>[12x]MAINFKGSPYLDRFDPSKDRTKVLFNPDRPLQQAELNEMQSIDQYYLKNLGDAIFKDGDKQSGLGFTLSEDNVLTVNPGYVYINGKIRYYDNDDSVKITGVGKETIGIKLTERIVTPDEDASLLDQTSGVPSYFSKGADRLEEKMSLTVNDPTSATIYTFMDGDLYIQSTNAEMDKINKVLAERTYDESGSYKVNGFELFSEGNAEDDDHVSVVVDAGKAYVKGFKVDKPVSTRISVPKSYDLGTAENESTIFNKSNNSISLANSPVKEIRRVTGQVLIEKERVTRGAQGDGQDFLSNNTAFEIVKVWTETSPGVTTKEYKQGEDFRLTDGQTIDWSPQGQEPSGGTSYYVSYKYNKRMEAGKDYEVTTQGEGLSKKWYINFTPSNGAKPIDQTVVLVDYTYYLARKDSVFINKYGDIAILPGEPNIMRLVTPPLNTDPENLQLGTVTVLPDSDEAVCISFAITRLSMEDLQKVKTRVDNLEYNQAVNALDDGAMEGQNPLTLRSVFSEGFISLDKADITHPDFGIVFSFEDAEATLAYTEAVNQPKIIPGDTTAHIWGRLISAPFTEERTIYQGQASETLNVNPYNIPNKQGVLKLTPSEDNWIDTENVTITEQKTKKVTMKRFWRHNESYYGETEHYLYSNLQLDAGQKWKGETYAYDREHGRTGTLLESGGQRTLEEMIEFIRIRDVSFEVKGLNPNDNNLYLLFDGVRCAITPATGYRKGSEDGTIMTDAKGTAKGKFTIPAGIRCGNREVTLKNANSTSATTYTAQGRKKTAQDIIIRTRVTVNLVDPLAQSFQYDENRTISSLGLYFASKGDKQSNVVIQIRGMGDQGYPNKTIYAETVMNADDIKVSNNASAETRVYFDDPMMAEGGKEYAIVIITENSDYTMWVGTRTKPKIDKPNEVISGNPYLQGVLFSSSNASTWTPHQNSDLKFGIYTSKFNETATIEFEPIKDVSADRIVLMSTYLTPERTGCTWEMKLILDDMASSTTFDQLKWEPIGNYQDLDVLGLARQVKLRATFESNRYISPLMSSSDLTFTTFLTELTGSYVGRAIDMTEAPYNTVRFSYEAFLPKGTKVVPKYSADDGKTWKTFTKSPTTTRANNEFTRYVIDEKVKSSGTNTKLQVRLDLSTENSFLRPRVRRLMVTTRDE;>[6x]MALNFTTITENNVIRDLTTQVNNIGEELTKERNIFDITDDLVYNFNKSQKIKLTDDKGLTKSYGNITALRDIKEPGYYYIGARTLATLLDRPDMESLDVVLHVVPLDTSSKVVQHLYTLSTNNNQIKMLYRFVSGNSSSEWQFIQGLPSNKNAVISGTNILDIASPGVYFVMGMTGGMPSGVSSGFLDLSVDANDNRLARLTDAETGKEYTSIKKPTGTYTAWKKEFEPKDMEKYLLSSIRDDGSASFPLLVYTSDSKTFQQAIIDHIDRTGQTTFTFYVQGGVSGSPMSNSCRGLFMSDTPNTSSLHGVYNAIGTDGRNVTGSVVGSNWTSPKTSPSHKELWTGAQSFLSTGTTKNLSDDISNYSYVEVYTTHKTTEKTKGNDNTGTICHKFYLDGSGTYVCSGTFVSGDRTDTKPPITEFYRVGVSFKGSTWTLVDSAVQNSKTQYVTRIIGINMP;>MAFNYTPLTETQKLKDMYPKVNDIGNFLKTEVNLSDVKQISQPDFNNILASIPDSGNYYVTNSKGAPSGEATAGFVRLDKRNVNYYKIYYSPYSSNKMYIKTYANGTVYDWISFKLDEGSLYNEGNTLNVKELTESTTQYATLVNPPKENLNTGWVNYKESKNGVSSLVEFNPVNSTSTFKMIRKLPVQEQKPNLLKDSLFVYPETSYSNIKTDNWDTPPFWGYSSNSGRSGVRFRGENTVQIDDGSDTYPSVVSNRFKMGKELSVGDTVTVSVYAKINDPALLKDNLVYFELAGYDTVDDTSKNPYTGGRREITASEITTEWKKYSFTFTIPENTIGASGVKVNYVSLLLRMNCSSSKGNGAVVYYALPKLEKSSKVTPFITHENDVRKYDEIWSNWQEVISKDELKGHSPVDIEYNDYFKYQWWKSEVNEKSLKDLAMTVPQGYHTFYCQGSIAGTPKGRSIRGTIQVDYDKCDPYRANKFVKLLFTDTEGIPYTLYYGGYNQGWKPLKQSETSTLLWKGTLDFGSTEAVNLNDSLDNYDLIEVTYWTRSAGHFSTKRLDIKNTSNLLYIRDFNISNDSTGSSVDFFEGYCTFPTRTSVQPGMVKSITLDGSTNTTKVASWNEKERIKVYNIMGINRG[6x];> MATDKEAKDVIDKFIDNVFNFDVLTKERIKEKDEEIKKITTDDMYEKVVYIRPYVGVIQSLNPQHVQYESFSNNGYDIEAELSFRKVSYLVDKGSIPTDSLSTLTVHLVERNQELLIDYFDEIQDVLYGEYMEEEYVFDEDVPLSTILALDLNDNLKSLSNIKYMFKGAPKENPFGTDKDVYIDTYNLLYWLYLGEDEELAYPMNINYFFTEGRFFTIFGKGHKYKVDVSKFIVGDILFFGRSDTNIGIYVGDGEFISMMGKFPKDETPIGKYKLDDYWNEFNGRVMRFDEEVYI;> MVVRFQSSMGRSLKRVDSD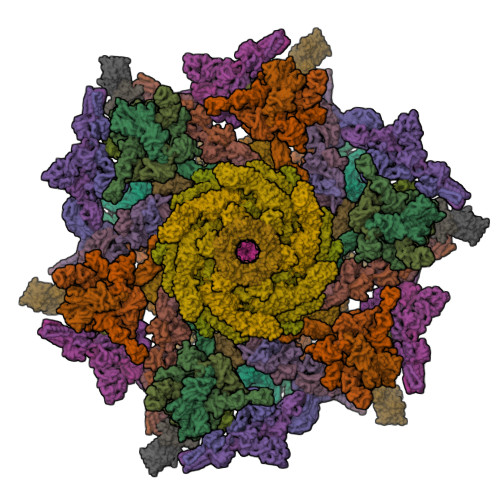DLNVKGLVLATVSKINYKYQSVEVKVNNLTLGSRIGDDGSLAVPYPKSFIGRTPEGSVFGTKPLITEGSVVLIGFLNDDINSPIILSVYGDNEQNKMINTNPLDGGKFDTESVYKYSSSLYEILPSLNYKYDDGEGTSIRTYNGKSFFSMTSGEEEKPQATDFYTGTEYQDLFTSYYGNKTLIEPRIQKAPNMLFKHQGVFYDDGTPDNHITTLFISERGDIRASVLNTETQKRTTQEMSSDGSYRVIKQDDDLMLDEAQVWIEYGISEDNKFYIKNDKHKFEFTDEGIYIDDKPMLENLDESIAEAMKNLNEIQKELDDINYLLKGVGKDNLEELIESTKESIEASKKATSDVNRLTTQIAEVSGRTEGIITQFQKFRDETFKDFYEDASTVINEVNQNFPTMKTDVKTLKTKVDNLEKTEIPNIKTRLTELENNNNNADKIISDRGEHIGAMIQLEENVTVPMRKYMPIPWSKVTYNNAEFWDSNNPTRLVVPKGITKVRVAGNVLWDSNATGQRMLRILKNGTYSIGLPYTRDVAISTAPQNGTSGVIPVKEGDYFEFEAFQDSEGDRQFRADPYTWFSIEAIELETETMEKDFMLIGHRGATGYTDEHTIKGYQMALDKGADYIELDLQLTKDNKLLCMHDSTIDRTTTGTGKVGDMTLSYIQTNFTSLNGEPIPSLDDVLNHFGTKVKYYIETKRPFDANMDRELLTQLKAKGLIGIGSERFQVIIQSFARESLINIHNQFSNIPLAYLTSTFSESEMDDCLSYGFYAIAPKYTTITKELVDLAHSKGLKVHAWTVNTKEEMQSLIQMGVDGFFTNYLDEYKKI;>MKTRKLTNILSKLIDKTMAGTSKITDFTPGSASRSLLEAVSLEIEQFYILTKENIDWGIQEGIIEAFDFQKRQSKRAYGDVTIQFYQPLDMRMYIPAGTTFTSTRQEYPQQFETLVDYYAEPDSTEIVVEVYCKETGVAGNVPEGTINTIASGSSLIRSVNNEYSFNTGTKEESQEDFKRRFHSFVESRGRATNKSVRYGALQIPDVEGVYVYEETGHITVFAHDRNGNLSDTLKEDIIDALQDYRPSGIMLDVTGVEKEEVNVSATVTISNKSRIGDTLQKHIESVIRSYLNNLKTSDDLIITDLIQAIMNIDDVLIYDVSFDNLDENIIVPPQGIIRAGEIKVELK[4x];> MRRIRRPKVRIEIVTDDNTFTLRFEDTRDYNGDEFGAKLLGFQTKNSMEDDSSVFQINMAGDTYWDKLVMANDIIRIFITPNDDPNDKEGKQERLIQVGMVSQVSKVGSYGNDQTQFRITGQSFVKPFMKFGLGVIQEVQAVLPEVGWLIDGDGDNEVKFTGSSAHEVMTGIIRRFIPYMKYNYTEKTYNTIDNYLDYDDLSSWDEFEKLTEVSAFTNFDGSLKQLMDMVTARPFNELFFKNSEKTPGKAQLVLRKTPFNPTEWRALDMIKVPTEDFIEEDVGKSDVETYSIFTATPAGMLKELNGDVFSKPQFHPELTDRYGYTKFEVENIYLSTKSGSATEDSDSSGDDNGTERGTYSKIMKDLSNYGRDNISKGIDKYTSKLSSKYKNLKKAQAKKIIEKFVKEGKVTEKEYEKITGNKVDDELTSDNRPKLTKDKLKSILKEKFKTQDDFNNSKKKKKAKTDALKELTTKYRFGNKTHATTLLDEYIKYKGEPPNDEAFDKYLKAIEGVSNVATDTGSDASDSPLVMFSRMLFNWYHGNPNFYAGDIIVLGDPKYDLGKRLFIEDKQRGDTWEFYIESVEHKFDYKQGYYTTVGVTRGLKDAILEDGKGSPHRFAGLWNQSSDFMGGLMGEDTSKELKEKGVAEKQSSGDKDGGSDSGGAQDGGSLDSLKKYNGKLPKHDPSFVQPGNRHYKYQCTWYAYNRRGQLGIPVPLWGDAADWIGGAKGAGYGVGRTPKQGACVIWQRGVQGGSPQYGHVAFVEKVLDGGKKIFISEHNYATPNGYGTRTIDMSSAIGKNAQFIYDKK;>MNNFIPQPQGLLRFLNTLDTDLTSSHMNLLDEEVSFVSKFYTPQLQLSELAKKVLTNIKTDDIPVLEREFNDNTIIHKANDTLLKVQAPRMYMILQSIVLEAYAIVNCFVENPSSLKYLTEEDVSITRENLNYVADYLGNYDDYNSVVLDLRDLDLCFSAIELQLPLIKKEANV[2x];>[2x]MANFLKNLHPLLRRDRNKKDNQDPNFALIDALNEEMNQVEKDAIESKLQSSLKTSTSEYLDKFGDWFGVYRKTDEKDDVYRARIIKYLLLKRGTNNAIIDAIKDYLGRDDIDVSVYEPFTNIFYTNKSHLNGEDHLMGYYYRFAVINVSIGDYFPVEIIDVINEFKPAGVTLYVTYDGASTIRGGAIIKWLDGLPKIETYQEFDRFTGYDDTFYGHINMNQSKDTDNSSSDIFKTNHSLINSLDVLTGSSSVGRQYINYGYVTSYVYNPGMTSSVNQISASTEGRGQEVPTDYYMYTSTKNNNTVELSMQTTSGVSYLYNNFNFRDYMSKYRPQVDLQSDEARRIVSDYIKELSIDYYLSAVIPPDESIEIKLQVYDFSINRWLTVSINNLSFYEKNIGSNIGYIKDYLNSELNMFTRLEINAGKRDSVDIKVNYLDLMFYYYERGIYTIKPYKALIENYLDISRETYVEAFKIASLSNGDIITKTGFQPIGYLKLVGNYENTIPSTINIVAKDTDNNPIESNELDVYNTVENRNLLQSYKGVNTIAREITSTKEFTVSGWAKEIYSTNYLSKVLKPGKVYTLSFDMEITGNDPTLKSYSDNHGIYLYSNTKGIVVNGVKSMERTIGNKVSVTQTFTAPTITDHRLLIYTGRYTSDGKASTPPVFFNTVKITELKLTEGSSKLEYSPAPEDKPNVIEKGIKFNNILTNIQTLSINSDTILKNVTLYYSYYGDSWVELKTLGNISTGETTETNNLIDLYGLQTVDYSNINPMSKVSLRSIWNVKLGELNNQEGSLSNMPNDYFNAVWQDIDKLSDIELGSMRMVKDTEGGVFDGATGEIIKATLFNVGAYTDLDMLAYTLTNYTEPLTLGSSRLISELKEELLTSESFNVDNRIKVIDSIYEELPNTSIIKNGFVEREVTGSKYLDYGLYEPIEDGTRYKLIVEGEFKDNIEFISLYNSNPNFNETFIYPSEIINGVAEKEFIAKPSTEDKPRLNTDVRIYIRPYDSTISKVRRVELRKV;>MRFKKHVVQHEETMQAIAQRYYGDVSYWIDLVEHNNLKYPYLVETDEEKMKDPERLASTGDTLIIPIESDLTDVSAKEINSRDKDVLVELALGRDLNITADEKYFNEHGTSDNILAFSTNGNGDLDTVKGIDNMKQQLQARLLTPRGSLMLHPNYGSDLHNLFGLNIPEQATLIEMEVLRTLTSDNRVKSANLIDWKIQGNVYSGQFSVEIKSVEESINFVLGQDEEGIFALFE[2x];>MPQSDGISNLHRIALRFPKEGGGYDMYRFKVNPENYTIDSPQRTTAIKTKSDIVIEDYGKDIEVINFTGTTGFRPVREADGLKTGKQKMEELQSRVSEYAMQGGSGNVSGSYLQFFNFTDDSYYKVHLAPQGLKITRSKDEPLLFRYEITLVVIGSLTEADRSAVTTEEFGNVKPNASQRVDEGIKELDKNARKTRDRNNQEISRRENTIPKSTGDNTNEGNRLKQSFPSSSIYNPRQSTNGLKGNIDNMALIIGYGDGGVSS[2x];>MAVEPFPRRPITRPHASIEVDTSGIGGSAGSSEKVFCLIGQAEGGEPNTVYELRNYSQAKRLFRSGELLDAIELAWGSNPNYTAGRILAMRIEDAKPASAEIGGLKITSKIYGNVANNIQVGLEKNTLSDSLRLRVIFQDDRFNEVYDNIGNIFTIKYKGEEANATFSVEHDEETQKASRLVLKVGDQEVKSYDLTGGAYDYTNAIITDINQLPDFEAKLSPFGDKNLESSKLDKIENANIKDKAVYVKAVFGDLEKQTAYNGIVSFEQLNAEGEVPSNVEVEAGEESATVTATSPIKTIEPFELTKLKGGTNGEPPATWADKLDKFAHEGGYYIVPLSSKQSVHAEVASFVKERSDAGEPMRAIVGGGFNESKEQLFGRQASLSNPRVSLVANSGTFVMDDGRKNHVPAYMVAVALGGLASGLEIGESITFKPLRVSSLDQIYESIDLDELNENGIISIEFVRNRTNTFFRIVDDVTTFNDKSDPVKAEMAVGEANDFLVSELKVQLEDQFIGTRTINTSASIIKDFIQSYLGRKKRDNEIQDFPAEDVQVIVEGNEARISMTVYPIRSFKKISVSLVYKQQTLQA[6x];>[6x]MASEAKQTVHTGNTVLLMIKGKPVGRAQSASGQREYGTTGVYEIGSIMPQEHVYLRYEGTITVERLRMKKENFADLGYASLGEEILKKDIIDILVVDNLTKQVIISYHGCSANNYNETWQTNEIVTEEIEFSYLTASDKART;>[12x]MAIATYNSHVELAKYLVSKADSVYLTIGKSTPWSNETNPPQPDENATVLQEVIGYKKATKVTLVRPSKSPEDDNKNLISYGNKSWVEVTPENAKAEGAKWVYLESSIVGDELPLGTYRQVGFVMDLVAKSGISKFNLVPSEVESTGTLLFFDNKQFQNRSEQTTAKERFIVEVDPNSSSVDKLAAALEHHHHHH> GMGDSAGLPPIYADKPIELAPAKIITSFPVNTFLENLASAPDGTIFVTNHEVGEIVSITPDGNQQIHATVEGKVSGLAFTSNGDLVATGWNADSIPVVSLVKSDGTVETLLTLPDAIFLNGITPLSDTQYLTADSYRGAIWLIDVVQPSGSIWLEHPMLARSNSESVFPAANGLKRFGNFLYVSNTEKMLLLRIPVDSTDKPGEPEIFVEQTNIDDFAFDVEGNLYGATHIYNSVVRIAPDRSTTIIAQAEQGVIGSTAVAFGQTEGDCTAIYVVTNGGMFLPPPTGVVPANVVRLEVGK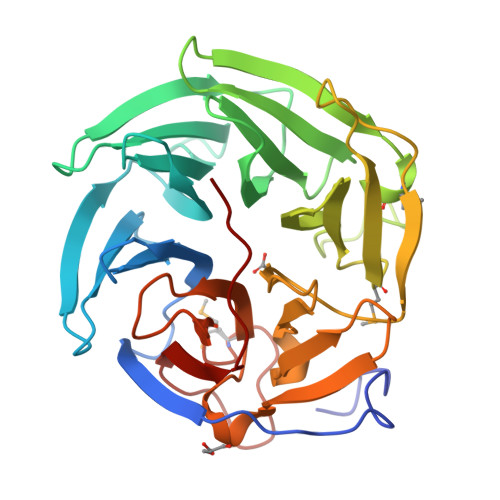PGYPLG>MIVKRPVSASLARAFFYIVLLSILSTGIALLTLASSLRDAEAINIAGSLRMQSYRLGYDLQSGSPQLNAHRQLFQQALHSPVLTNLNVWYVPEAVKTRYAHLNANWLEMNNRLSKGDLPWYQANINNYVNQIDLFVLALQHYAERKMLLVVAISLAGGIGIFT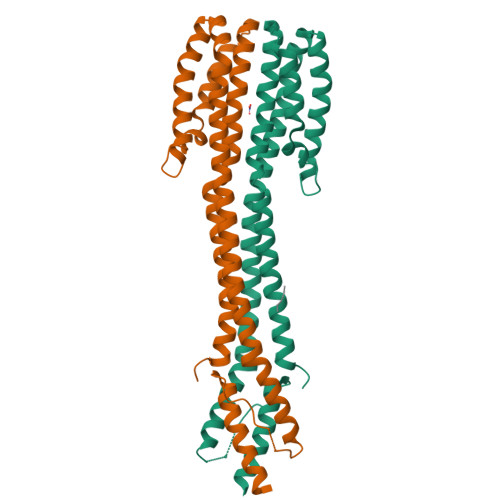LVFFTLRRIRHQVVAPLNQLVTASQRIEHGQFDSPPLDTNLPNELGLLAKTFNQMSSELHKLYRSLEHHHHHH[2x]>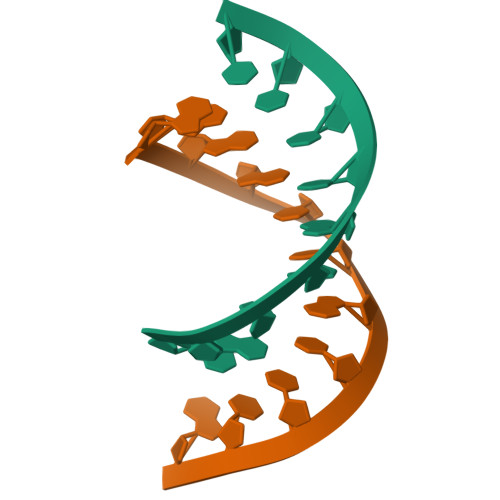CAGUGGUCUU[4x];>[4x]AAGACUGCCUG>[2x]APDTSVSNKQNFSTDVIYQIFTDRFSDGNPANNPTGAAFDGTCTNLRLYCGGDWQGIINKINDGYLTGMGVTAIWISQPVENIY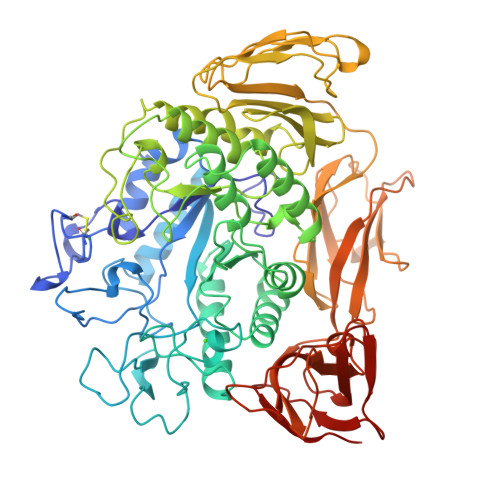SIINYSGVNNTAYHGYWARDFKKTNPAYGTIADFQNLIAAAHAKNIKVIIDFAPNHTSPASSDQPSFAENGRLYDNGTLLGGYTNDTQNLFHHNGGTDFSTTENGIYKNLYDLADLNHNNSTVDVYLKDAIKMWLDLGIDGIRMDAVKHMPFGWQKSFMAAVNNYKPVFTFGEWFLGVNEVSPENHKFANESGMSLLDFRFAQKVRQVFRDNTDNMYGLKAMLEGSAADYAQVDDQVTFIDNHDMERFHASNANRRKLEQALAFTLTSRGVPAIYYGTEQYMSGGTDPDNRARIPSFSTSTTAYQVIQKLAPLRKCNPAIAYGSTQERWINNDVLIYERKFGSNVAVVAVNRNLNAPASISGLVTSLPQGSYNDVLGGLLNGNTLSVGSGGAASNFTLAAGGTAVWQYTAATATPTIGHVGPMMAKPGVTITIDGRGFGSSKGTVYFGTTAVSGADITSWEDTQIKVKIPAVAGGNYNIKVANAAGTASNVYDNFEVLSGDQVSVRFVVNNATTALGQNVYLTGSVSELGNADPAKAIGPMYNQVVYQYPNWYYDVSVPAGKTIEFKFLKKQGSTVTWEGGSNHTFTAPSSGTATINVNWQP>MASGTTTTAVKIGIIGGTGLDDPEILEGRTEKYVDTPFGKPSDALILGKIKNVDCVLLARHGRQHTIMPSKVNYQANIWALKEEGCTHVIVTTACGSLREEIQPGDIVIIDQFIDRTTMRPQSFYDGSHSCARGVCHIPMAEPFCPKTREVLIETAKKLGLRCHSKGTMVTIEGPRFSSRAESFMFRT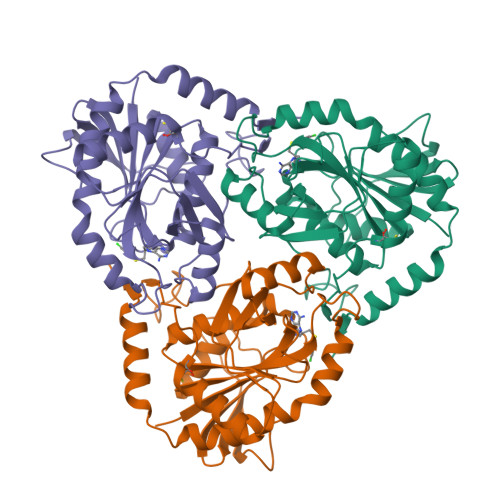WGADVINMTTVPEVVLAKEAGICYASIAMATDYDCWKEHEEAVSVDRVLKTLKENANKAKSLLLTTIPQIGSTEWSETLHNLKNMAQFSVLLPRH[2x]> 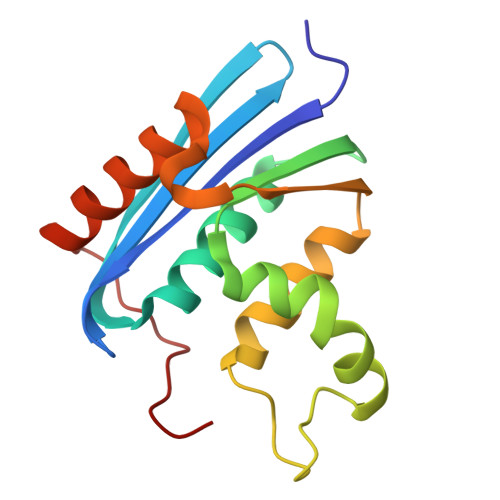MLKQVEIFTDGSCLGNPGPGGYGAILRYRGREKTFSAGYTRTTNNRMELMALIVALEALKEHCEVILSTDSQYVRQGITQWIHNWKKRGWKTADKKPVKNVDLWQRLDAALGQHQIKWEWVKGHAGHPENERCDELARAAAMNPTLEDTGYQVEV>MMGDLTTSFPATTLTTNDQPHVVVCSGAGMGHLTPFLNLASALSSAPYNCKVTLLIVIPLITDAESHHISSFFSSHPTIHRLDFHVNLPAPKPNVDPFFLRYKSISDSAHRLPVHLSALSPPISAVFSDFLFTQGLNTTLPHLPNYTFTTTSARFFTLMSYVPHLAKSSSSSPVEIPGLEPFPTDNIPPPFFNPEHIFTSFTISNAKYFSLSKGILVNTFDSFEPETLSALNSGDTLSDLPPVIPIGPLNELEHNKQEELLPWLDQQPEKSVLYVSFGNRTAMSSDQILELGMGLERSDCRFIWVVKTSKIDKDDKSELRKLFGEELYLKLSEKGKLVKWVNQTEILGHTAVG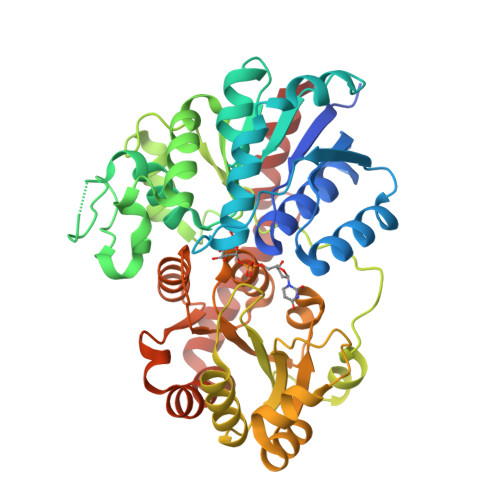GFLSHCGWNSVMEAARRGVPILAWPQHGDQRENAWVVEKAGLGVWEREWASGIQAAIVEKVKMIMGNNDLRKSAMKVGEEAKRACDVGGSSATALMNIIGSLKR[2x]> KVKMSGLITVRTNEPLGVEKIKEVISKALENIEQDYESLLNIKIYTIGAPRYRVDVVGTNPKEASEALNQII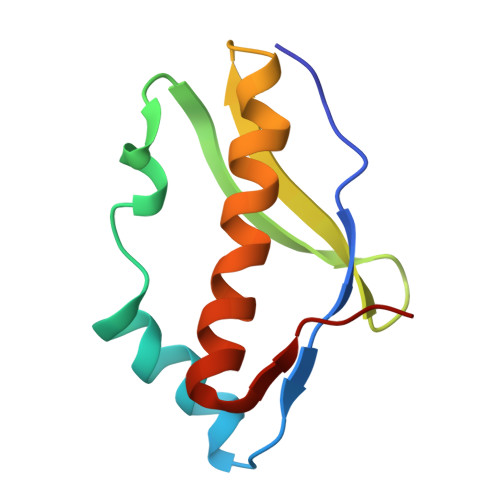SNLIKIGKEENVDISVV> AMPFEIEVLLPGELSPAETSALQKCEG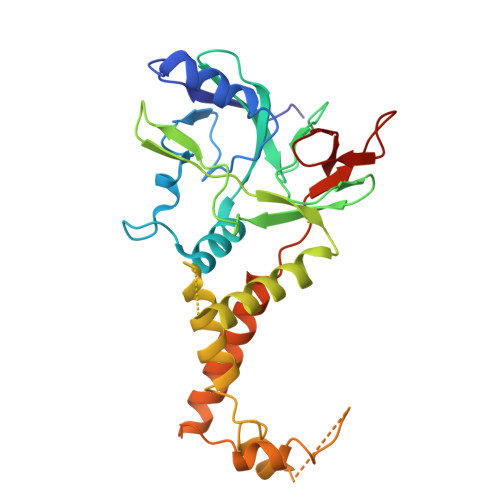KIITFSTLRHRASLVDIALSSYYINGAPPDTLSLLEAYRMRFAAVITRVIPGKLLAHAIGVGTPTPGLFIQNTSPVDLCNGDYICLLPPVYGSADSIRLDSVGLEIVFPLTIPQTLMREIIAKVVARAVEDLNLMFSINEGCLLILALIPRLLALLIPRLLALVTREAAQLIHPEAPMLMLPIYETISSWISTSSRLGDTLGTRAILRVCVFDGPSTVHPGDRTAVIQV> HHHHHHMGIEWIIRRSVANRFLVLMGALFLSIWGTWTIINTPVDALPDLSDVQVIIKTSYPGQAPQIVENQVTYPLTTTMLSVPGAKTVRGFSQFGDSYVYVIFEDGTDPYWARSRVLEYLNQVQGKLPAGVSAELGPDATGVGWIYEYALVDRSGKHDLADLRSLQDWFLKYELKTIPDVAEVASVGGVVKEYQVVIDPQRLAQYGISLAEVKSALDASNQEAGGSSIELAEAEYMVRASGYLQTLDDFNHIVLKASENGVPVYLRDVAKVQIGPEMRRGIAELNGEGEVAGGVVILRSGKNAREVIAAVKDKLETLKSSLPEGVEIVTTYDRSQLIDRAIDNLSGKLLEEFIVVAVVCALFLWHVRSALVAIISLPLGLCIAFIVMHFQGLNANIMSLGGIAIAVGAMVDAAIVMIENAHKRLEEWQHQHPDATLDNKTRWQVITDASVEVGPALFISLLIITLSFIPIFTLEGQEGRLFGPLAFTKTYAMAGAALLAIVVIPILMGYWIRGKIPPESSNPLNRFLIRVYHPLLLKVLHWPKTTLLVAALSVLTVLWPLNKVGGEFLPQINEGDLLYMPSTLPGISAAEAASMLQKTDKLIMSVPEVARVFGKTGKAETATDSAPLEMVETTIQLKPQEQWRPGMTMDKIIEELDNTVRLPGLANLWVPPIRNRIDMLSTGIKSPIGIK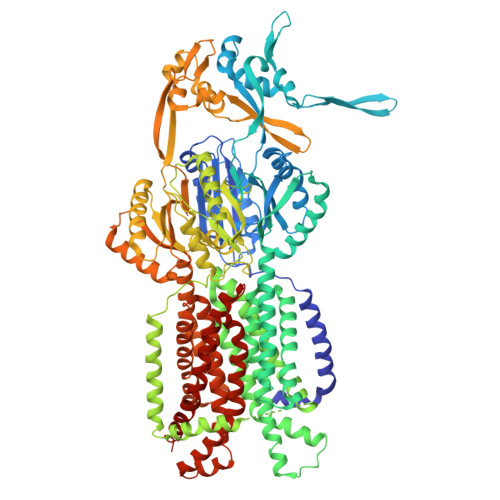VSGTVLADIDAMAEQIEEVARTVPGVASALAERLEGGRYINVEINREKAARYGMTVADVQLFVTSAVGGAMVGETVEGIARYPINLRYPQSWRDSPQALRQLPILTPMKQQITLADVADIKVSTGPSMLKTENARPTSWIYIDARDRDMVSVVHDLQKAIAEKVQLKPGTSVAFSGQFELLERANHKLKLMVPMTLMIIFVLLYLAFRRVGEALLIISSVPFALVGGIWLLWWMGFHLSVATGTGFIALAGVAAEFGVVMLMYLRHAIEAVPSLNNPQTFSEQKLDEALYHGAVLRVRPKAMTVAVIIAGLLPILWGTGAGSEVMSRIAAPMIGGMITAPLLSLFIIPAAYKLMWLHRHRVRK>MGSDKIHHHHHHMPHLFYGTAQNGEVIFDEREAHHMRVVRLKEGDVIEATDGNGFSYTCILKSLKKKTAAAKIVKVEEKEKEPTEKLSVVVPIGRWERTRFLIEKCVELGVDEIFFHKFERSQHEISLDKAKIVVREAAKQC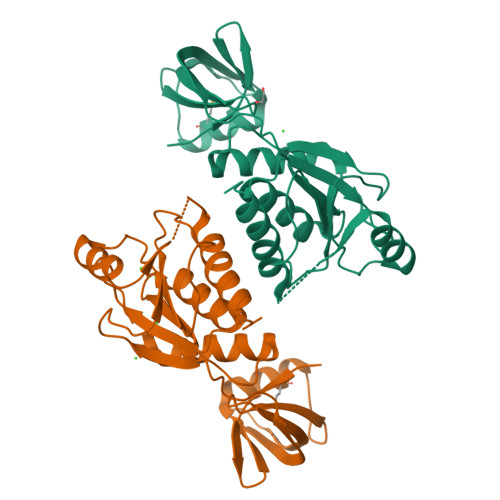KRYLFPKVSFLEKLEFSGNVITLDLDASQNLLDANLEGSITVVVGPEGGFSEKERELLRSSTTIVSLGKKILRFETAAILTVGYIALKKQKI[2x]>[2x]GG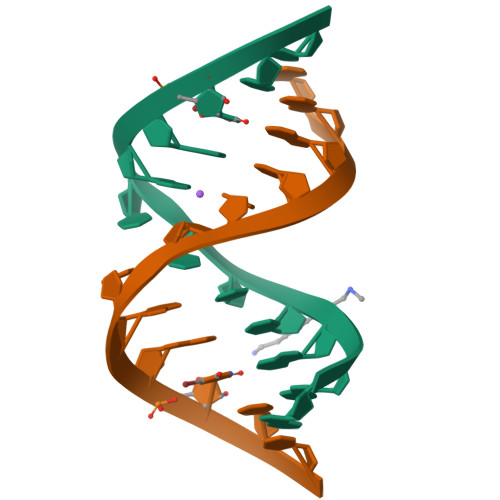ACUCCGGUCC>[4x]MTAARHEPHLLTDAVRAFQAQSPVWRPADDEEALRGLEAAELTVPLDYRAPAGRTLTLGLVRHRATAPERRRGVLLVGPGDDLGNRGTLLGAQLVGQLPKEVLAQYDVVAFDHRFMGRSSPVVCGLEPEERFWVFHHPRDFDHEVRFQANVAAKVAEHALDILPYASSRNIARDIEVIRGALGEDRISYLGYSYGTYLGAVWTQMFGEHADRVVLDSICSPDWVWRG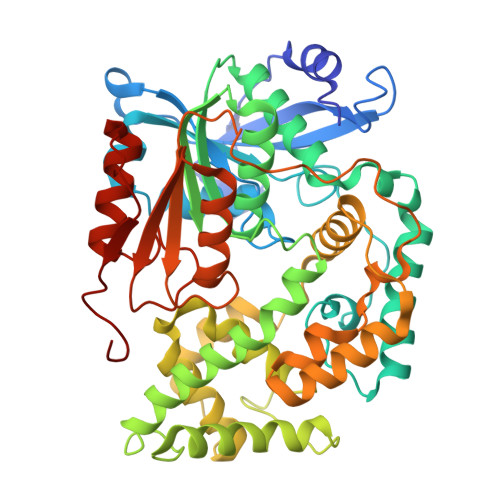LFTDFPPNGERALTRWARWAAARDADLGLGATDGAVRAAYDGVLARVDTDREVTVAGFPLDRTLARLIVVGMLNSDRNYPFLGDIVRSAVHGGQLEPATMGFLGQMFGQPKEESGTVAQLAILAGDWAWPRNVDLYERDMERASRTHPFTGAAMAGIKAPAFWPVPPSEPVTRLGPDNPADSILLVQAADDMSTPLAAARRMREVLGDTSRLLTVADTAHHRVFPFYGNPGADELVTAYLVDGELPAADVTRPNPAPMVPTV> GADKYIDTITGFS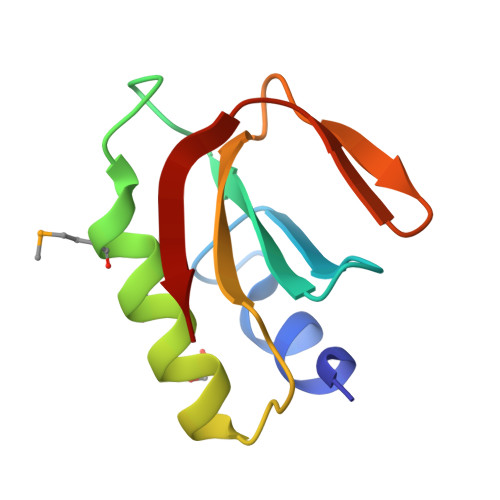CEKAAVTDNGFLVIAIDADSDSGYDMLASQFLEEAKKEGVSGLKGVLIVDIKNAKFEQGAVVGKRIGKAYK> MFKLSWIFGRKKDNAACSESAPEKVAQIPQHDPLDPMIKLGRIRGWNVEPEKAPVIRSVKDFLEPGLSVAMDSAYGDGPTPAAKAAAGGQNPYVVPTMLQDWYNSQGFIGYQACAIISQHWLVDKACSMSGEDAARNGWELKSDGRKLSDEQSALIARRDMEFRVKDNLVELNRFKNVFGVRIALFVVESDDPDYYEKPFNPDGITPGSYKGISQIDPYWAMPQLTAGSTADPSSEHFYEPDFWIISGKKYHRSHLVVVRGPQPPDILKPTYIFGGIPLTQRIYERVYAAERTANEAPL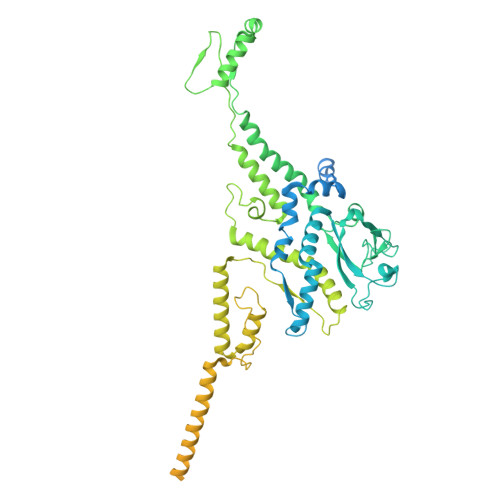LAMSKRTSTIHVDVEKAIANEDAFNARLAFWIANRDNHGVKVLGTDESMEQFDTNLADFDSIIMNQYQLVAAIAKTPATKLLGTSPKGFNATGEHETISYHEELESIQEHIFDPLLERHYLLLAKSEEIDVQLEIVWNPVDSTSSQQQAELNNKKAATDEIYINSGVVSPDEVRERLRDDPRSGYNRLTDDQAETEPGMSPENLAEFEKAGAQSAKAKGEAERAEAQAGAVEGAGDPVPAAPRGTKPLAKAAEEGASEAAEPPSRPDPKAELRNLLVDLLSKLQDLDDIKAPDGVDIEHNDAPGVKRTSKPGVSGMEPSVFSSNRIVGPRDHSELQRIKVNGITTLIENPRGSIRQGKDGSWRVQMKHHYGFIKGTKGADGDEVDCFVGPNLGSKRVFVVNQVNKEGQFDEHKCMLGFNNINDAKSGYLSCFRPGWDGLGSIHEVDLPAFRRWLANGDTTKPFGGE> NTEGDALYSLRQSLKDANNVLQSWDPTLVNPCTWFHVTCNTDNSVIRVDLGNAQLSGALVSQLGQLKNLQYLELYSNNISGTIPLELGNLTNLVSLDLYLNKFTGGIPDTLGKLLKLRFLRLNNNSL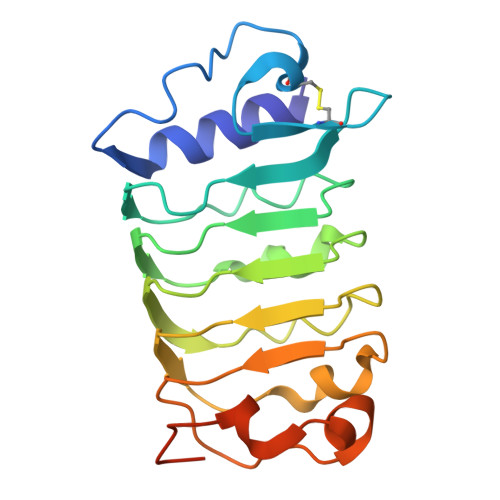SGQIPQSLTNISTLQVLDLSNNNLSGAVPSTGSFSLFTPISFGNNPNLCGPGTTKPCPGA>AGSGHMMELHILEHRVRVLSVARPGLWLYTHPLIKLLFLPRRSRCKFFSLTETPEDYTLMVDEEGFKELPPSEFLQVAEATWLVLNVSSHSGAAVQAAGVTKIARSVIAPLAEHHVSVLMLSTYQTDFILVREQDLSVVIHTLAQEFDIYREVGGEPVPVTRDDSSNGFPRTQHGPSPTVHPIQSPQNRFCVLTLDPETLPAIATTLIDVLFYSHSTPKEAASSSPEPSSITFFAFSLIEGYISIVMDAETQKKFPSDLLLTSSSGELWRMVRIGGQPLGFDECGIVAQIAGPLAAADISAYYISTFNFDHALVPEDGIGSVIEVLQRRQEGLAS[3x];> AGSGHMMELHILEHRVRVLSVARPGLWLYTHPLIKLLFLPRRSRCKFFSLTETPEDYTLMVDEEGFKELPPSEFLQVAEATWLVLNVSSHSGAAVQAAGVTKIARSVIAPLAEHHVSVLMLSTYQTDFILVREQDLSVVIHTLAQEFDIYREVGGEPVPVTRDDSSNGFPRTQHGPSPTVHPIQSPQNRFCVLTLDPETLPAIA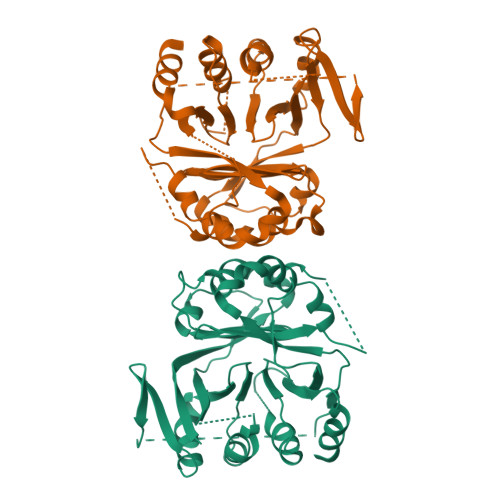TTLIDVLFYSHSTPKEAASSSPEPSSITFFAFSLIEGYISIVMDAETQKKFPSDLLLTSSSGELWRMVRIGGQPLGFDECGIVAQIIGPLAAADISAYYISTFNFDHALVPEDGIGSVIEVLQRRQEGLAS5-cyclohexylpentan-1-ol | C11 H22 O | 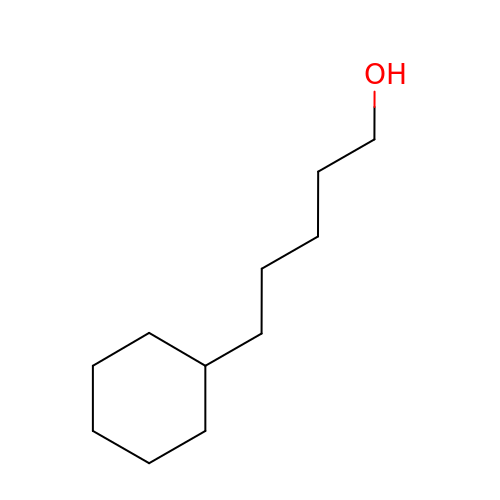DOUCFSUZXLHVHJ-UHFFFAOYSA-N> MSAEAADREAATSSRPCTPPQTCWFEFLLEESLLEKHLRKPCPDPAPVQLIVQFLEQASKPSVNEQNQVQPPPDNKRNRILKLLALKVAAHLKWDLDILEKSLSVPVLNMLLNELLCISKVPPGTKHVDMDLATLPPTTAMAVLLYNRWAIRTIVQSSFPVKQAKPGPPQLSVMNQMQQEKELTENILKVLKEQAADSILVLEAALKLNKDLYVHTMRTLDLLAMEPGMVNGETESSTAGLKVKTEEMQCQVCYDLGAAYFQQGST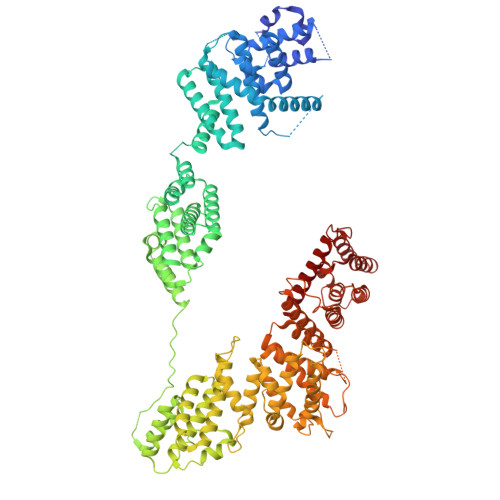NSAVYENAREKFFRTKELIAEIGSLSLHCTIDEKRLAGYCQACDVLVPSSDSTSQQLTPYSQVHICLRSGNYQEVIQIFIEDNLTLSLPVQFRQSVLRELFKKAQQGNEALDEICFKVCACNTVRDILEGRTISVQFNQLFLRPNKEKIDFLLEVCSRSVNLEKASESLKGNMAAFLKNVCLGLEDLQYVFMISSHELFITLLKDEERKLLVDQMRKRSPRVNLCIKPVTSFYDIPASASVNIGQLEHQLILSVDPWRIRQILIELHGMTSERQFWTVSNKWEVPSVYSGVILGIKDNLTRDLVYILMAKGLHCSTVKDFSHAKQLFAACLELVTEFSPKLRQVMLNEMLLLDIHTHEAGTGQAGERPPSDLISRVRGYLEMRLPDIPLRQVIAEECVAFMLNWRENEYLTLQVPAFLLQSNPYVKLGQLLAATCKELPGPKESRRTAKDLWEVVVQICSVSSQHKRGNDGRVSLIKQRESTLGIMYRSELLSFIKKLREPLVLTIILSLFVKLHNVREDIVNDITAEHISIWPSSIPNLQSVDFEAVAITVKELVRYTLSINPNNHSWLIIQADIYFATNQYSAALHYYLQAGAVCSDFFNKAVPPDVYTDQVIKRMIKCCSLLNCHTQVAILCQFLREIDYKTAFKSLQEQNSHDAMDSYYDYIWDVTILEYLTYLHHKRGETDKRQIAIKAIGQTELNASNPEEVLQLAAQRRKKKFLQAMAKLYF6,7-DIMETHYL-3-[(METHYL{2-[METHYL({1-[3-(TRIFLUOROMETHYL)PHENYL]-1H-INDOL-3-YL}METHYL)AMINO]ETHYL}AMINO)METHYL]-4H-CHROMEN-4-ONE 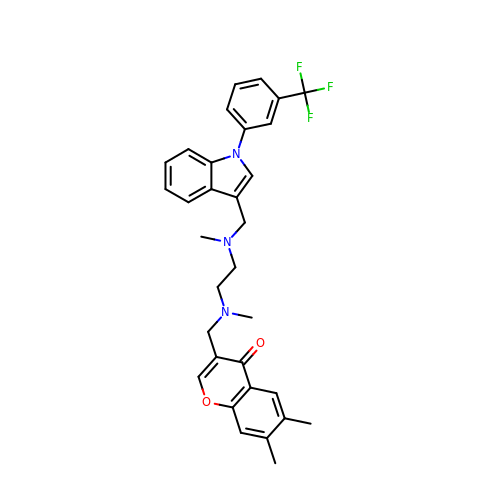| C32 H32 F3 N3 O2 | JZNXLPPJRFFECJ-UHFFFAOYSA-N>MGDTLTAGQKLERGGSLQSGNGAYTLTLQDDGNLVLYARDKAVWSTGTNGQDVVRAEVQTDGNFVLYTAEKPVWHTDTKGKKEVKLVLQDDRNLVLYAKDGPAWSLE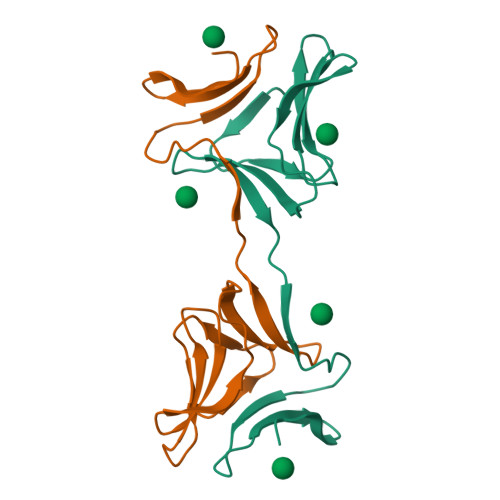HHHHHH[4x]> MLKIISANVNGIRSAYKKGFYEYIAASGTDIVCVQELKAQEADLSADMKNPHGMHGHWHCAEKRGYSGVAVYSKRKPDNVQIGM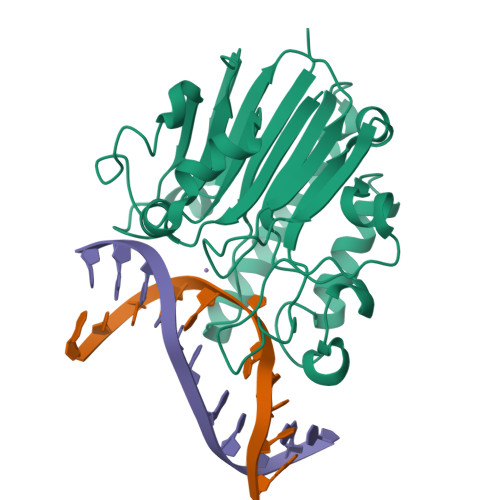GIEEFDREGRFVRCDFGRLSVISLYLPSGSSAEERQQVKYRFLDAFYPMLEAMKNEGRDIVVCGNWNIAHQNIDLKNWKGNQKNSGFLPEEREWIGKVIHKLGWTDMWRTLYPDVPGYTWWSNRGQAYAKDVGWRIDYQMVTPELAAKAVSAHVYKDEKFSDHAPLVVEYDYAAE> MSQSLEEKSVQERTRIKNSRYESGVIPYAKMGYWNPDYQVKDTDVLALFRVTPQPGVDPIEAAAAVAGESSTATWTVVWTDLLTAADLYRAKAYKVDQVPNNPEQYFAYIAYELDLFEEGSIANLTASIIGNVFGFKAVKALRLEDMRLPFAYIKTFQGPATGVILERERLDKFGRPLLGCTTKPKLGLSGKNYGRVVYEALKGGLDFVKDDENINSQPFMRWRERYLFVMEAVNKAAAATGEVKGHYLNVTAATMEEMYARAQLAKELGSVIIMIDLVIGYTAIQTMAKWARDNDMILHLHRAGNSTYSRQKNHGMNFRVICKWMRMAGVDHIHAGTVVGKLEGDPIITRGFYKTLLLPKLERNLQEGLFFDMDWASLRKVMPVASGGIHAGQMHQLIHYLGEDV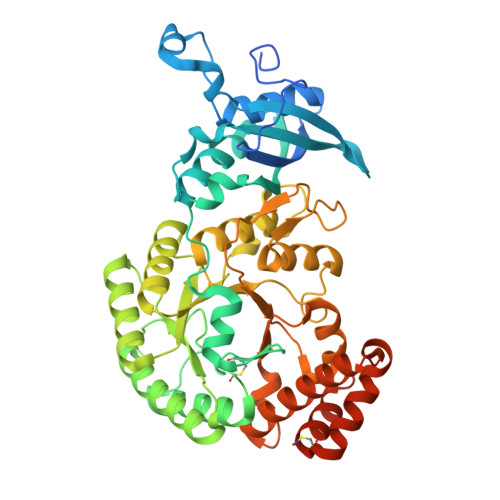VLQFGGGTIGHPDGIQSGATANRVALEAMILARNENRDFLTEGPEILREAAKNCGALRTALDLWKDITFNYTSTDTSDFVETPTANI> MGVISDAYRLKYTFGVDFGTSYVKYGPITLNEPKMVQTRGLFLRDLPESVKMRIPPDVLARGLVVGDEEVRKYLSSVRDVQRNLKYPLKDGVARRDDEEAWRVLKELARYTLAQFPVSDPEFAGWLVAVALSALAPDYMYKAIFDIYDELASEFKIYAVTILPQPLAVAIAENAVNCVIVEGGHGNIQVAPISFALIREGLVALNRGGAEANAITREILKDIGYSDIAREEYAVEVVKRAVGLVPRRLKEA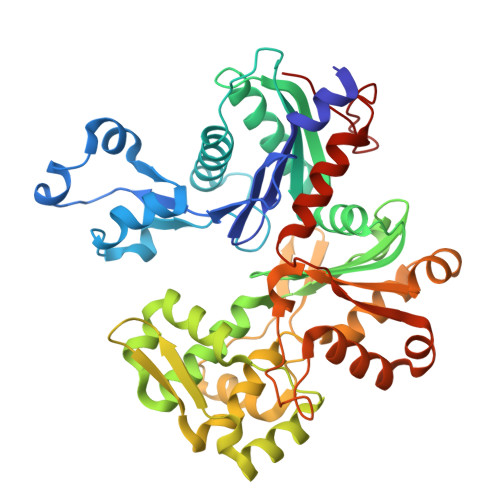IRAAKSDPDRFVTKVRLSPVVEVEIPREYAWTRFLIGEIVFDPNHEEIKSYIEQSRLRIENAVIGDVTLYGEMDVASAIITSLRNVSVEIQERVASQIILSGGAFSWRVPPGMEDVAADSVTRVKIALEEKSPALASKVEVRLVSEPQYSVWRGAVIYGYALPLSLEWSDTTREGWRFPRR>SLSEDKMDLYLQQG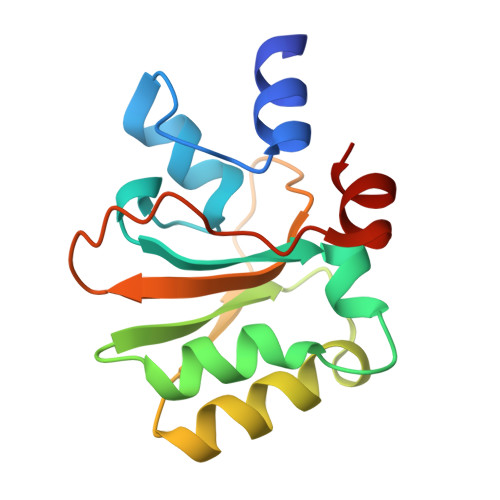MYGPLETKPDERHLFLGSLRERVVLALTKGQVLRSKPYKEAEHELKNSHNVTLLINGELQYQSYSSYIQMASRYGVPFKIVSDLQFHTPLGIVIAADIAVNRELIYIQDDIYNRSVLKS[2x]> VLEATMILIDNSEWMINGDYIPTRFEAQKDTVHMIFNQKINDNPENMCGLMTIGDNSPQVLSTLTRDYGKFLSAMHDLPVRGNAKFGDGIQIAQ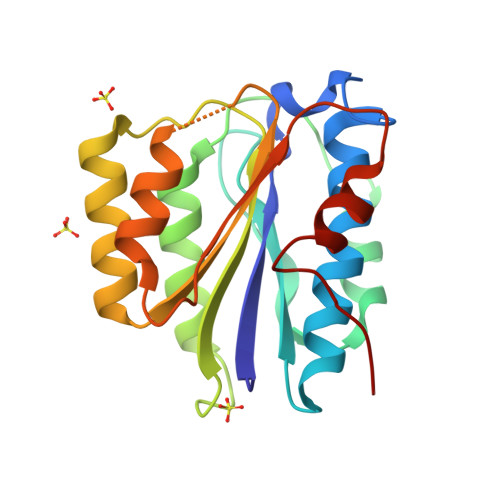LALKHRENKIQRQRIVAFVGSPIVEDEKNLIRLAKRMKKNNVAIDIIHIGELQNESALQHFIDAANSSDSCHLVSIPPSPQLLSDLVNQSPIGQGVVA4,5-DE-EPOXYPIMARICIN | C33 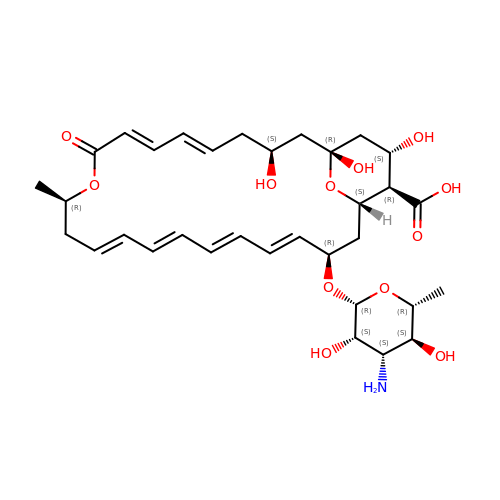H47 N O12 | SQKHCBHOKICFHY-FNNGFRNWSA-N> GIPRNSSTGAKTAKSDKLKVVATNSIIADMTKAIAGDKIDLHSIVPIGQDPHEYEPLPEDAEKTSNADVIFYNGINLEDGGQAWFTKLVKNAQKTKNKDYFAVSDGIDVIYLEGASEKGKEDPHAWLNLENGIIYSKNIAKQLIAKDPKNKETYEKNLKAYVAKLEKLDKEAKSKFDAIAENKKLIVTSEGCFKYFSKAYGVPSAYIWEINTEEEGTPDQISSLIEKLKVIKPSALFVES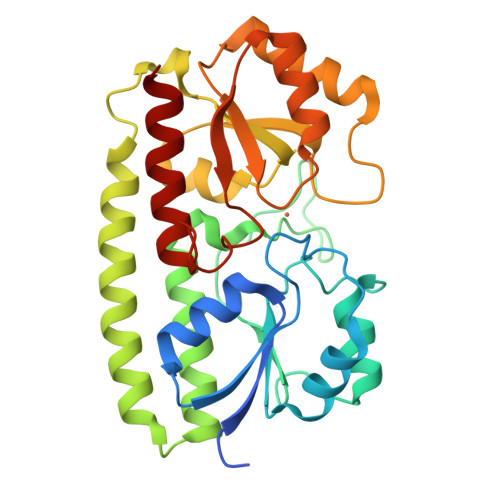SVDRRPMETVSKDSGIPIYSEIFTDSIAKKGKPGDSYYAMMKWNLDKISEGLAK[(2R,3S,4R,5R)-5-(2,4-dioxo-3,4-dihydropyrimidin-1(2H)-yl)-3,4-dihydroxytetrahydrofuran-2-yl]methyl (2R,5S,6R)-3,3,4,4-tetrafluoro-5-hydroxy-6-(hydroxymethyl)tetrahydro-2H-pyran-2-yl dihydrogen 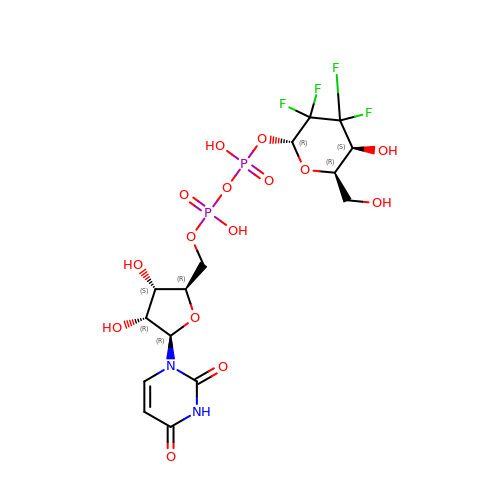diphosphate (non-preferred name) | C15 H20 F4 N2 O15 P2 | MUYRTPUNBLMMOR-UMEAPJPCSA-N Here, we show that A. baumannii Slam secretes HphA, which functions as a hemophore that acquires heme from hemoglobin and albumin. HphA is composed of a C-terminal 8-stranded β-barrel packed against an N-terminal clamp-like structure through 6 intermediate β-strands. Once secreted, HphA has the dual capacity of binding hemoglobin and scavenging heme. HphA along with its cognate receptor, HphR, function together as a two-component receptor required for full virulence and facilitating extrapulmonary dissemination and/or survival in the blood.

To examine the heme-binding potential of HphA, acid-acetone extraction was used to strip the co-purifying heme. The resulting apo protein is devoid of heme and refolds to its native conformation as indicated by the absence of a Soret signature in the UV–Vis spectra and X-ray crystal structures. Apo HphA also crystallized in a C2221 space group, with three monomers in the asymmetric unit. All apo HphA chains adopt an open conformation and do not show structural heterogeneity in the heme-binding region. Comparison of holo and apo structures reveals that the loop containing H43 undergoes a large conformational change upon heme binding and release, while the 310 helix containing H106 is only slightly displaced. Size exclusion chromatography-multi-angle light scattering (SEC-MALS) confirmed that HphA exists as a monomer in solution, regardless of the presence of heme. Apo HphA interacts specifically with hemoglobin conjugated to agarose beads as evidenced by pull-down. Based on the pull-down results, we propose that apo HphA binds to Hb largely through its heme-Fe coordination residues, H43 and H106. This mode of binding is plausible as the loop containing H43 is flexible and could wedge itself into the heme-binding site, positioning HphA to capture spontaneously released heme using H106 in a relatively quick step. The loop containing H43 then dissociates from Hb and clamps down on heme in a relatively slower binding step.

>MGSSHHHHHHSGIDGISSNESNIKIGAAANASHPGGVAAVSVQAAGAPYNAFTGFSSLKGLAQAFAAQGTSNTNVTVGSKTFNISHIPVSAMPPSHSALGNFNFGQVGTQEVYFGEWWKAGDTPASASHTVYYAGDNTNTTVPTAGTATYTVAGINGSGSNLLSGTFTANYGAGTLEGTLTGTGTAVSSLSLDGVAFNPGTAAFAGLATANGTAGIDNSGVVQGQFFGANASALAGIAQFDNVSYNTAFGGAKN[3x]> A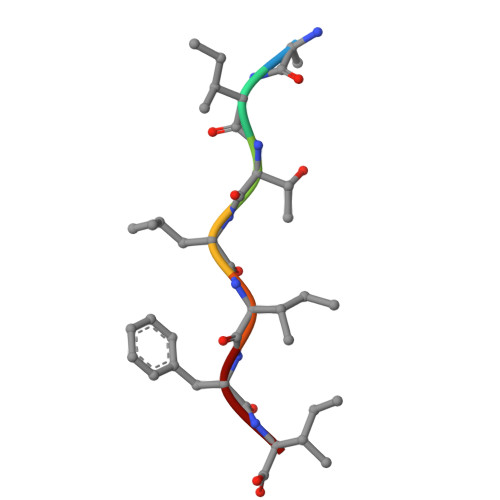ITLIFI> SSMEIRVRVEKDPELGFSISGGVGGRGNPFRPDD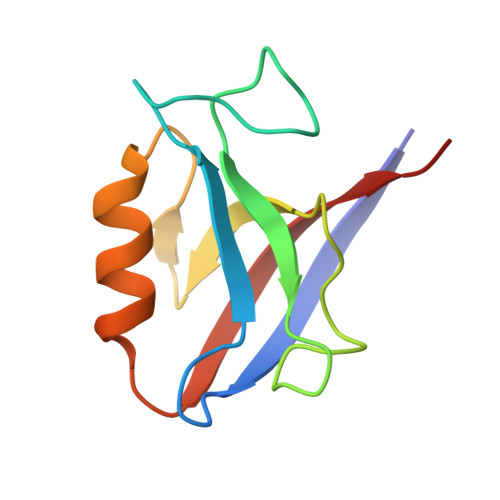DGIFVTRVQPEGPASKLLQPGDKIIQANGYSFINIRLEEAERLLKTFQNTVELIIVREVSS>[2x]ADSDVPNDILEEQLYNSIVVADYDSAVEKSKHLYEEKKSEVITNVVNKLIRNNKMNCMEYAYQLWLQGSKDIVRDCFPVEFRLIFAENAIKLMYK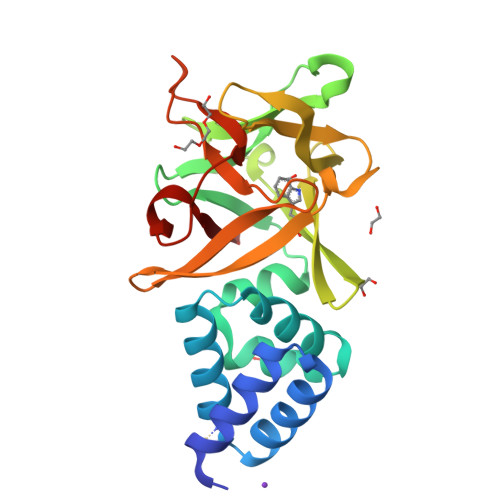RDGLALTLSNDVHGNDGRLAFGDGKDKTSPKVSWKFIALWENNKVYFKILNTERNQYLVLGVGTNPNGDHMAFGVNSVDSFRAQWYLQPAKYDKDNLFYIYNREYSKALTLSRTLETSGNRMAWGYNGRVIGSPEHYAWGVKAF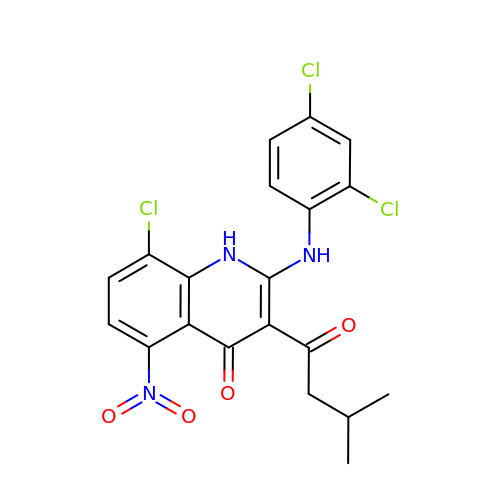8-chloro-2-[(2,4-dichlorophenyl)amino]-3-(3-methylbutanoyl)-5-nitroquinolin-4(1H)-one | C20 H16 Cl3 N3 O4 | LRTXIQCBQIKIOH-UHFFFAOYSA-N> MALQLSREQGITLRGSAEIVAEFFSFGINSILYQRGIYPSETFTRVQKYGLTLLVTTDLELIKYLNNVVEQLKDWLYKCSVQKLVVVISNIESGEVLERWQFDIECDKTAKDDSAPREKSQKAIQDEIRSVIAQITATVTFLPLLEVSCSFDLLIYTDKDLVVP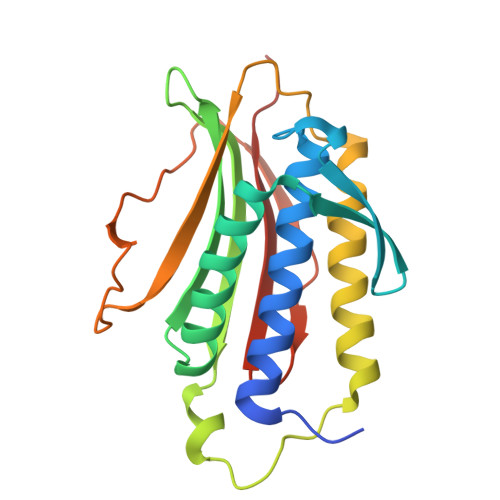EKWEESGPQFITNSEEVRLRSFTTTIHKVNSMVAYKIPVND(10E)-hexadec-10-en-12-yn-1-ol | C16 H28 O | 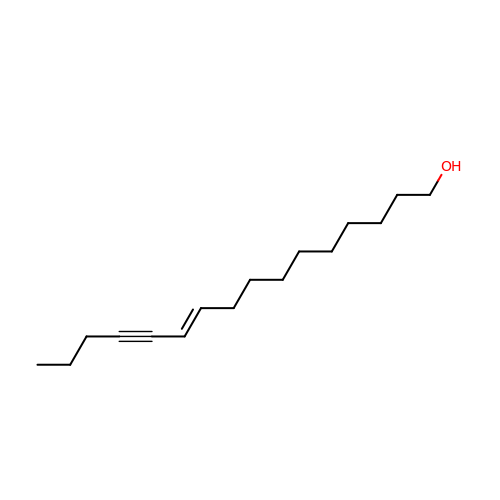CVGZIQCJXLSQQU-VOTSOKGWSA-N> DDNGIVLLGERAAKCRAYAKALHYKELEFQKGPTPAILESLISINNKLQQPEAAAGVLEYAMKHFGELEIQATWYEKLHEWEDALVAYDKKMDTNKDDPELMLGRMRCLEALGEWGQLHQQCCEKWTLVNDETQAKMARMAAAAAWGLGQWDSMEEYTCMIPRDTHDGAFYRAVLALHQDLFSLAQQCIDKARDLLDAELTAMAGESYSRAYGAMVSCHMLSELEEVIQYKLVPERREIIRQIWWERLQGCQRIVEDWQKILMVRSLVVSPHEDMRTWLKYASLCGKSGRLALAHKTLVLLLGVDPSRQLDHPLPTVHPQVTYAYMKNMWKSARKIDAFQHMQHFVQTMQQQAQHAIATEDQQHKQELHKLMARCFLKLGEWQLNLQGINESTIPKVLQYYSAATEHDRSWYKAWHAWAVMNFEAVLHYKHQNQARDEKKKLRHASGANITNATTAATTAATATTTASTEGSNSESEAESTENSPTPSPLQKKVTEDLSKTLLMYTVPAVQ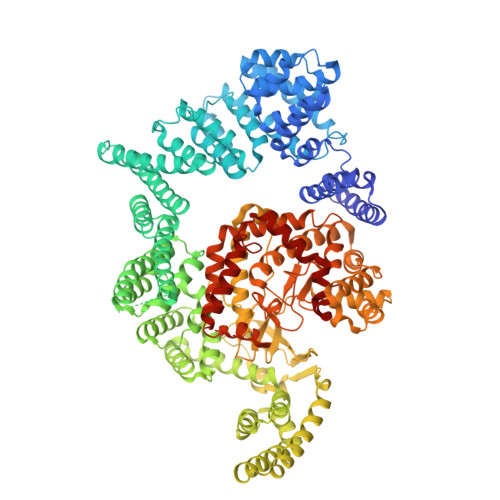GFFRSISLSRGNNLQDTLRVLTLWFDYGHWPDVNEALVEGVKAIQIDTWLQVIPQLIARIDTPRPLVGRLIHQLLTDIGRYHPQALIYPLTVASKSTTTARHNAANKILKNMCEHSNTLVQQAMMVSEELIRVAILWHEMWHEGLEEASRLYFGERNVKGMFEVLEPLHAMMERGPQTLKETSFNQAYGRDLMEAQEWCRKYMKSGNVKDLTQAWDLYYHVFRRISKQLPQLTSLELQYVSPKLLMCRDLELAVPGTYDPNQPIIRIQSIAPSLQVITSKQRPRKLTLMGSNGHEFVFLLKGHEDLRQDERVMQLFGLVNTLLANDPTSLRKNLSIQRYAVIPLSTNSGLIGWVPHCDTLHALIRDYREKKKILLNIEHRIMLRMAPDYDHLTLMQKVEVFEHAVNNTAGDDLAKLLWLKSPSSEVWFDRRTNYTRSLAVMSMVGYILGLGDRHPSNLMLDRLSGKILHIDFGDCFEVAMTREKFPEKIPFRLTRMLTNAMEVTGLDGNYRITCHTVMEVLREHKDSVMAVLEAFVYDPLLNWRLMDTNTKGNKRSRTRTDSYSAGQSVEILDGVELGEPAHKKTGTTVPESIHSFIGDGLVKPEALNKKAIQIINRVRDKLTGRDFSHDDTLDVPTQVELLIKQATSHENLCQCYIGWCPFW>[4x]SLIEDARKEREAAVAAAAAAVPSE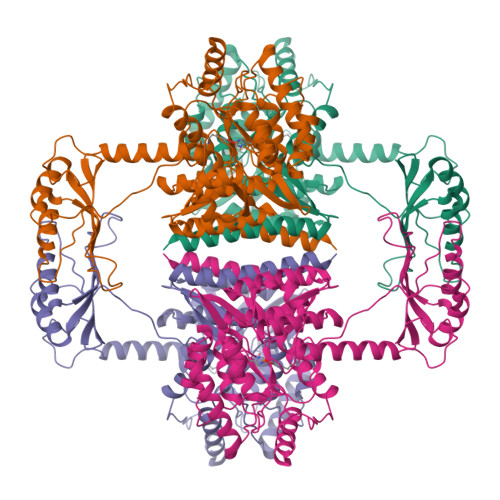PGDPLEAVAFEEKEGKAMLNLLFSPRATKPSALSRAVKVFETFEAKIHHLETRPAQRPRAGGPHLEYFVRLEVRRGDLAALLSGVRQVSEDVRSPAGPKVPWFPRKVSELDKCHHLVTKFDPDLDLDHPGFSDQVYRQRRKLIAEIAFQYRHGDPIPRVEYTAEEIATWKEVYTTLKGLYATHACGEHLEAFALLERFSGYREDNIPQLEDVSRFLKERTGFQLRPVAGLLSARDFLASLAFRVFQCTQYIRHASSPMHSPEPDCCHELLGHVPMLADRTFAQFSQDIGLASLGASDEEIEKLSTLYWFTVEFGLCKQNGEVKAYGAGLLSSYGELLHCLSEEPEIRAFDPEAAAVQPYQDQTYQSVYFVSESFSDAKDKLRSYASRIQRPFSVKFDPYTLAIDVLDSPQAVRRSLEGVQDELDTLAHALSAIG>[2x]MTIQDFQSSGKATVLAVGTAV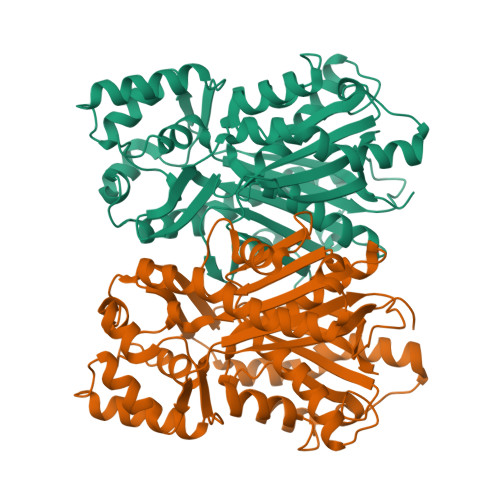PPKEFDQSTYPDFYFNVTNCNDKVELKGKFQRICDRSGIKKRHFYLDEEILKANPGMCTYMGASLDVRQNIAVREVPKLAKEAALKAIKEWGQPKSKITHLVFGTTSGVDMPGADFQLLKLLGLRPNVKRIMLYQQGCSAGATVTRVAKDLAENNPGARVLVACSEVTAVTFRAPSETHLDGLVGAALFGDGAAALIIGSNPTPVEKPLFEVHWSGQCVLPDSDGAILGHLREAGLVFHLLKDVPGIISKNIEKLLAEPLDYVKSVDEASPAYTDLFWVVHPGGPAILDQVEAKLKLDKDRMQATRDVLAQYGNMSSASVLFVLDQMRKRSVELNKDTTGDGLKWGVMLGFGPGLTVETLLLKSI> GSTGSPP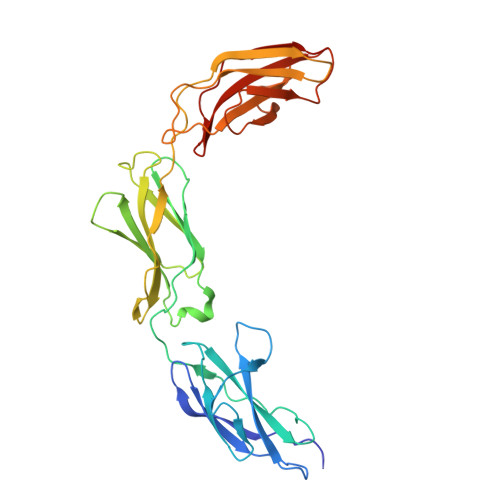GPPTSIHVEEITDTTATLSWRPGPDNHSPITAYTIQARTPFSLGWQAVSTVPEVVGGSHLTATVIELNPWVEYEFRVLASNAVGTGEPSKPSKKARTKDTVPKVTPANVSGGGGSRSELVITWEPVPEELQNGAGFGYVVAFRPFGSTGWMQAAVPSPEASKYVFKNETILPFSPFQVKVGAYNNKGEGPFGPVITIYSAEEEPGRAPSRLRAKSLSASDVEVSWKALPWSTSKKRVLGYELRYWEKNEKEDASSVLRTVGNRTLAIIQGLKGSSTYYITVRAYNTAGTGPPSPVVNITTKK> MSVQIGNGLLMVVAPGTLTVGSARARLIRQVTLADFCEPQAERPGLVVLALRHPADLAGAAYAATPPGKNHRDLEEAWLALDEGGRGLGGDGIRASVVSLNFLVAAAENADDALRAHVTTNYRDRRTAARLERFATVLRAMIRSHVFPHRALHVLGGLLGHVTQDRLASVTCVARGDQEAARTNDMAARRSQVHVPACALMDVDRELR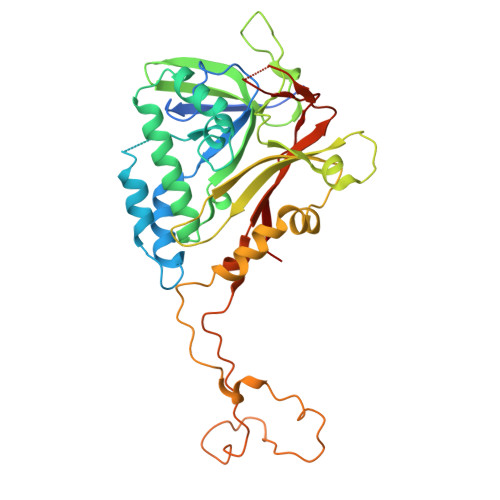LGGDDGLRFAYLVFVYTQRHRREALRVHVAVSRLPELGDALSFLLAGTRVDNAIHGTDEADAPAAPAAAAAFPAYLFNDPRSARCPTGRLNTPAAEALPVWAPDMRGRATRNSCMYAAYVRLGTVERVVRRAERCGSVDLPLAHMERFTWDVGAWEECFF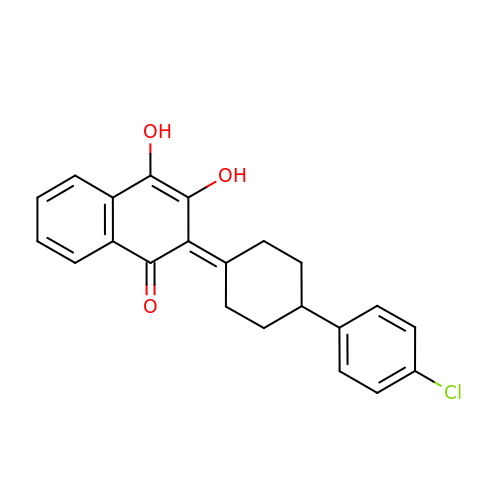2-[4-(4-CHLOROPHENYL)CYCLOHEXYLIDENE]-3,4-DIHYDROXY-1(2H)-NAPHTHALENONE | C22 H19 Cl O3 | HKIDMHSZRQSXJE-RNMGOYHCSA-N>[2x]GG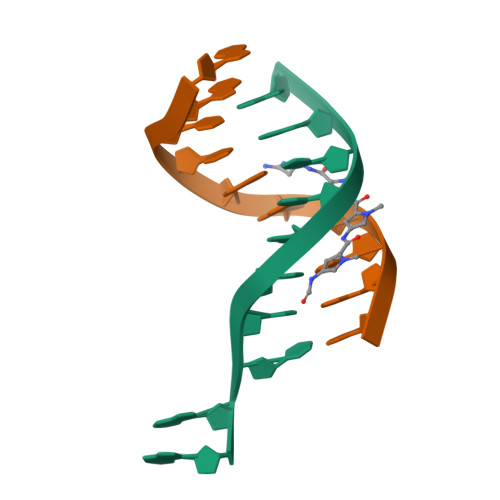CCAATTGG> PISPIETVPVKLKPGMDGPKVKQWPLTEEKIKALVEICTEMEKEGKISKIGPENPYNTPVFAIKKKDSTKWRKLVDFRELNKRTQDFWEVQLGIPHPAGLKKKKSVTVLDVGDAYFSVPLDEDFRKYTAFTIPSINNETPGIRYQYNVLPQGWKGSPAIFQSSMTKILEPFRKQNPDIVIYQYMDDLCVGSDLEIGQHRTKIEELRQHLLRWGLTTPDKKHQKEPPFLWMGYELHPDKWTVQPIVLPEKDSWTVNDIQKLVGKLNWASQIYPGIKVRQLCKLLRGTKALTEVIPLTEEAELELAENREILKEPVHGVYYDPSKDLIAEIQKQGQGQWTYQIYQEPFKNLKTGKYARMRGAHTNDVKQLTEAVQKITTESIVIWGKTPKFKLPIQKETWETWWTEYWQATWIPEWEFVNTP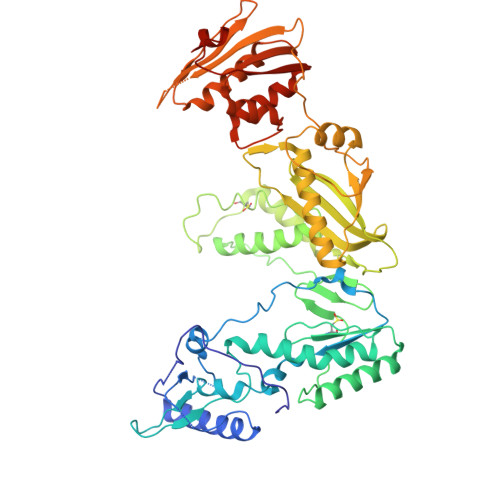PLVKLWYQLEKEPIVGAETFYVDGAANRETKLGKAGYVTNRGRQKVVTLTDTTNQKTELQAIYLALQDSGLEVNIVTDSQYALGIIQAQPDQSESELVNQIIEQLIKKEKVYLAWVPAHKGIGGNEQVDKLVSAGIRKVL>[2x]ARRPTICFRPINPSDLERLEQ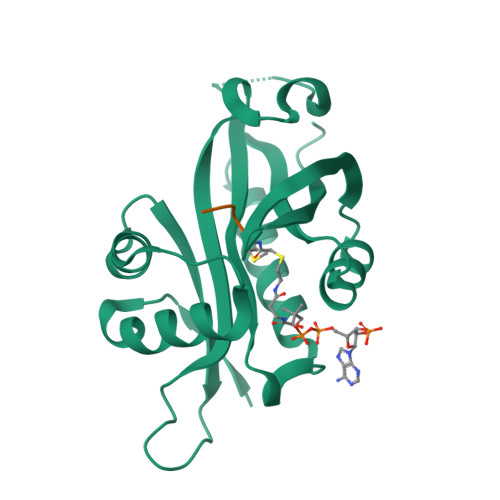IHRDIFPIRYESEFFQNVVNGGDIVSWAAVDRSRPDGHSEELIGFVTAKIVLAKESEISDLIRYDSSKGEGTLVYILTLGVVETYRKRGIAKALINEVVKYSSGIPVCRGVYLHVIAHNNPAIRLYKRMSFRCVRRLHGFYLINGQHFDSYLFVYFINGS;>MVNA[2x]> GSHMASEITSLDTENIDEILNNADVALVNFYADWCRFSQMLHPIFEEASDVIKEEFPNENQVVFARVDCDQHSDIAQRYRISKYPTLKLFRNGMMMKREYRGQRSVKAL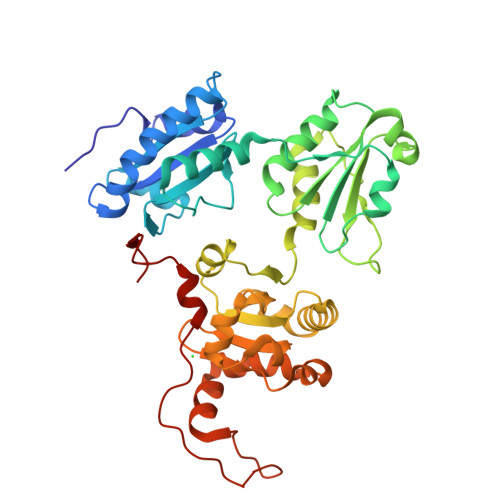ADYIRQQKSDPIQEIRDLAEITTLDRSKRNIIGYFEQKDSDNYRVFERVANILHDDCAFLSAFGDVSKPERYSGDNIIYKPPGHSAPDMVYLGAMTNFDVTYNWIQDKCVPLVREITFENGEELTEEGLPFLILFHMKEDTESLEIFQNEVARQLISEKGTINFLHADCDKFRHPLLHIQKTPADCPVIAIDSFRHMYVFGDFKDVLIPGKLKQFVFDLHSGKLHREFHHGPDPTDTAPGEQAQDVASSPPESSFQKLAPSEYRYTLLRD>[2x]MDAQYDISFADVEKAHINIRDSIHLTPVLTSSILNQLTGRNLFFKCELFQKTGSFKIRGALNAVRSLVPDALERKPKAVVTHSSGNHGQALTYAAKLEGIPAYIVVPQTAPDCKKLAIQAYGASIVYCEPSDESRENVAKRVTEETEGIMVHPNQEPAVIAGQGTIALEVLNQVPLVDALVVPVGGGGMLAGIAITVKALKPSVKVYAAEPSNADDCYQSKLKGKLMPNLYPPETIADGVKSSIGLNTWPIIRDLVDDIFTVTEDEIKCATQLVWERMKLLIEPTAGVGVAAVLSQHFQTVSPEVKNICIVLSGGNVDLTSSITWVKQAERPASYQSVSVHHHHHHQ

Human serine racemase (hSR) catalyses racemisation of L-serine to D-serine, the latter of which is a co-agonist of the NMDA subtype of glutamate receptors that are important in synaptic plasticity, learning and memory. In mammals, D-serine is synthesised by a pyridoxal-5′-phosphate (PLP)-containing enzyme serine racemase (SR). The first mammalian structures of SR, published in 201031, revealed a dimeric structure with each subunit consisting of a small domain (residues 78–153) and a large domain (residues 4–67 and 156–316). The roles of Ser 84 and Lys 56 as the Si and Re-face acid/bases in the catalytic cycle of hSR are generally accepted.

In this paper we describe the first ‘closed’ crystal structure of hSR bound to ATP. In this structure, Tyr 121 has ‘flipped’ outwards from the core of the small domain, where it is situated in the holoenzyme structures, to form H-bonds with the α-phosphate of ATP at the dimer interface. There is a radical change in conformation of the side-chain of Tyr 121 between the malonate/ATP complex and the holo structure, with the side-chain hydroxyl group ‘moving’ approximately 10 Å from interacting with the α-phosphate of ATP to the main-chain carbonyl of Ser 84. Malonate resides in the substrate binding site with Ser 84 pointing towards the central carbon; in the transition state this carbon is planar (see quinonoid intermediate). The binding site for ATP is in a pocket between the two subunits. The adenine ring sits between Ala A117 (from the α5 helix in the small domain of the A-subunit) and Arg B277 from the large domain of the B-subunit. Residues from both the large and small domains of the A-subunit make a number of hydrogen bonds to oxygens on the ribose and the α-phosphate of ATP. The β and γ phosphates of the ATP interact with the B-subunit, accepting hydrogen bonds from residues at the N-terminus of the α2 helix (main-chain NHs from Ser B32 and Ile B33, and sidechain OHs from Ser B31 and Ser B32). A magnesium ion, coordinated by two oxygens from the β and γ phosphates of the ATP and four waters, does not directly contact the protein but helps orient the β and γ phosphates of the ATP, facilitating the interaction with the N-terminus of the α2-helix from subunit B. In the malonate/ATP ‘closed’ complex, the C-terminal residues are better ordered and Trp 325 has good density and reasonable temperature factors.(4S,6R)-4-[2,4-difluoro-5-({[1-(trifluoromethyl)cyclopropyl]amino}methyl)phenyl]-4,6-dimethyl-5,6-dihydro-4H-1,3-thiazin-2-amine | 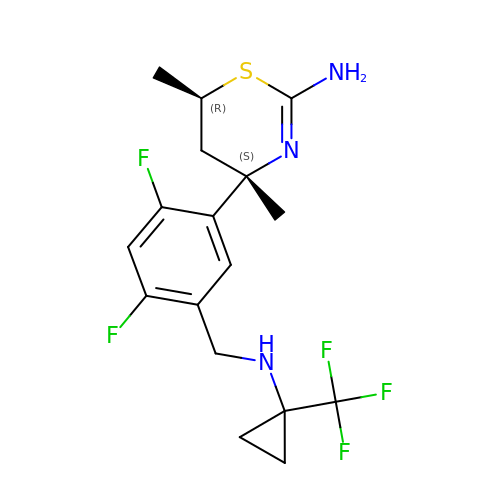C17 H20 F5 N3 S | ZQULGQNNJUBPOZ-PSLIRLAXSA-N>[4x]GSHMSDNNATDILFVGGIDETIDEKSLYDIFSSFGDIRNIEVPLNM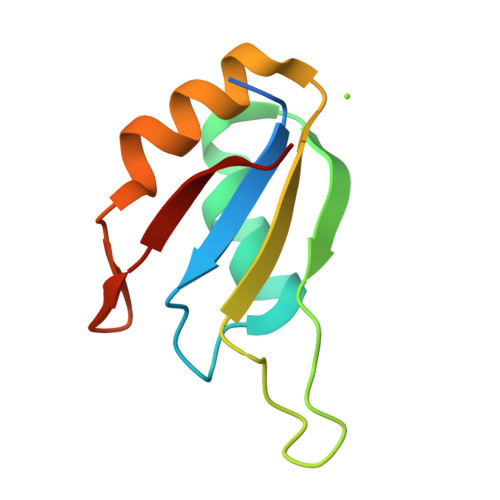TTKKNRGFAFVEYVEVDDAKHALYNMNNFELNGKRIHVNYSKT>GSHMASMKKKGSVVIVGRINLSGDTAYAQQTRGEEGCQETSQTGRDKNQVEGEVQIVSTATQTFLATSINGVLWTVYHGAGTRTIASPKGPVTQMYTNVDKDLVGWQAPQGSRSLTPCTCGSSDLYLVTRHADVIPVRRRGDSRGSLLSPRPISYLKGSAGGPLLCPAGHAVGIFRAAVSTRGVAKAVDFIPVESLETTMRSP[4x];>SECTT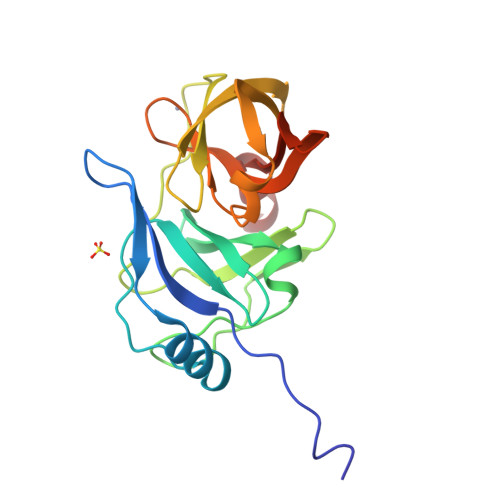PC[3x]> MELLDAVNTCLT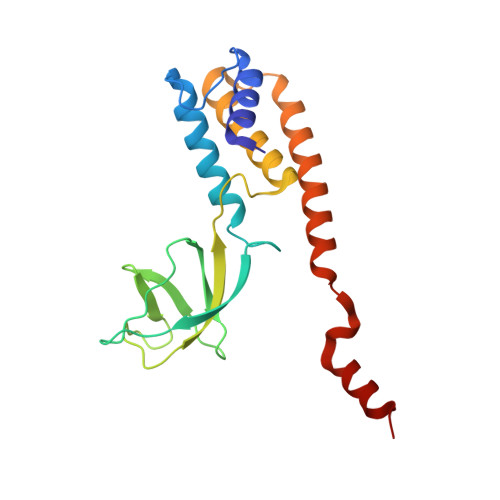ALGEARVTSTDTRHPSVALILQTLATKQKLLLERGWWFNTQDEEMFPDLLGRIPYPAASISVESLDGYNIYSKRNNFLFNNTCNTMYFTGPVCIRVTYNLDFEDLPESVATVITYRAARAVYVGDLGNDASVQDLVLNEQQAMLLVEEQHMRNKKHSTRRRRPWGKYQNALSG> QDSTSDLIPAPPLSKVPLQQNFQDNQFHGKWYVVGEAGNSLLRED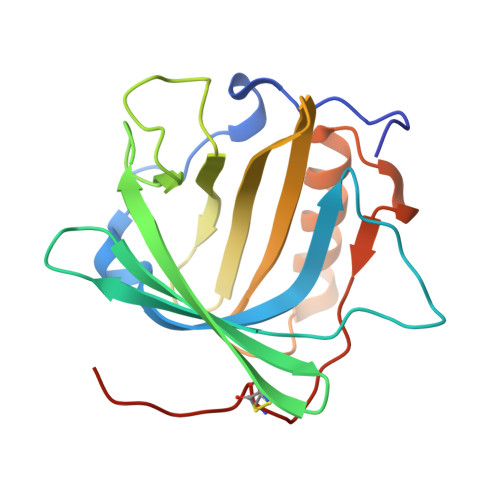KDPRKMYATIYELKEDKSYNVTSVRFRSKKCHYLIRTFVPGSQPGEFTLGLIKSKPGHTSFLVRVVSTNYNQHAMVFFKTVAQNREYFFITLYGRTKELTSELKENFIRFSKSLGLPENHIVFPVPIDQCIDGSAWSHPQFEK> GSHMERYDIAIIGSGPAGLASAINAKTRNKSVIVFGSSDLSKKLTLAPVINNYLGFYGIRGAELQEKFKEHIDNMGIQIENVKVNNIYAMGEYFSIMTSKDTYEASKVILAMGMEHTKPLKGEDKFLGRGVGYSATCDAPLYKGKIVTIVGYNKEAESEANYLAELASKV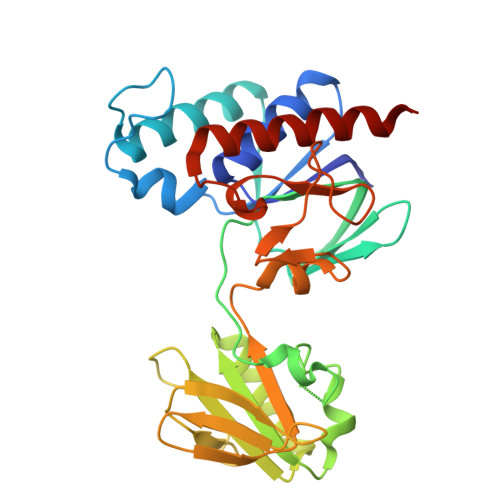YYVPRYKDEYQLVSAVEIVKDVPVEIVGDKKVEKLKLKSRELETDGVFVLKDSAPPEQLVPGLYVEDGHIKVNRKMETNIDGCYAAGDCTGKPYQYMKAVGEGQVAALNAVEKLYTKA> ETQVVLINAVKDVAKALGDLISAT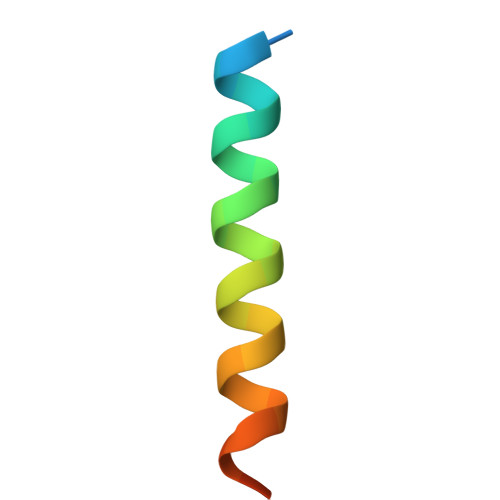KAAAG>[2x]SNAFNGVSEAELLTKTLPDILTFNLDIVIIGINPGLMAAYKGHHYPGPGNHFWKCLFMSGLSEVQLNHMDDHTLPGKYGIGFTNMVERTTP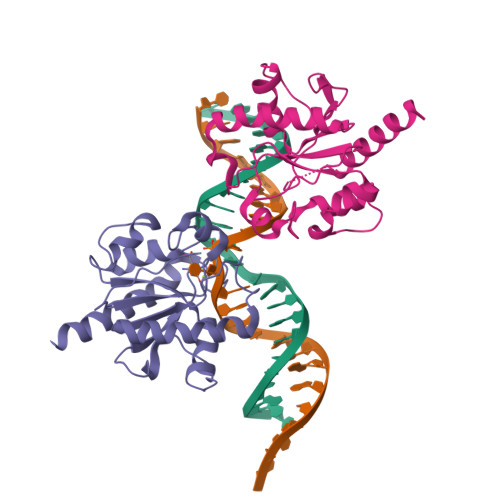GSKDLSSKEFREGGRILVQKLQKYQPRIAVFNGKCIYEIFSKEVFGVKVKNLEFGLQPHKIPDTETLCYVMPSSSARCAQFPRAQDKVHYYIKLKDLRDQLKGIERNMDV>[4x]MGSSHHHHHHSSGLVPRGSHMASAPAAVVQEVSAEAQAPAVVKNPPKLALKIDRADVNQLPRNFRMGSDKYVGVTKTGIMPTRKGMDTMNVSASSCFSEKELEAILKKVPVKPSQFYDVDLRGESHGYLNGTAVSWFANHDWGNDGRTEDIIIPLEKEQLASLKGSTVKSIYRFDDKKNVILSPVYVNYNKVRTEEEMVKQHGANYFRLTLQDHFRPDDPDVDKFLEFYKSLPKDAWLHYHSYAGMGRTTIFMVMHDILKNAKDVSFDDIIQRQKLIGIVDLSEIPDKKKNYGRKAYIERYQFVQHFYDYVKENPDLKTPYSVWAKKNKVNSWEPDYNGYIWRLDTKDRNQLPRNFRTMNSAFRTDVNVKKTGKGFTPTPTRKGLDTLYMSGSAEFSNGELQAMLPVLKQQAKGP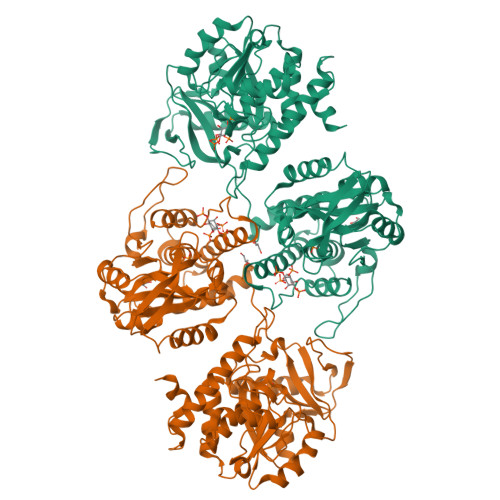IYIMDLRQETHGVFNGNAVSWYGLRDWGNLGKNKAEVLKDENSRLNAARGKSLIVAELDKDKMPIDPKPVKIESVMTEQQLVEKNGLHYYRIAATDHIWPSAANIDEFINFTRTMPANAWLHFHSQAGAGRTTAYMAMYDMMKNPDVSLGDILSRQYLLGGNYVAYEIAKPKPDQWKADYYHQKAHMIEKFYQYVQENHADGFKTSWSQWLAAHQDV> EERKKELAKEVIETA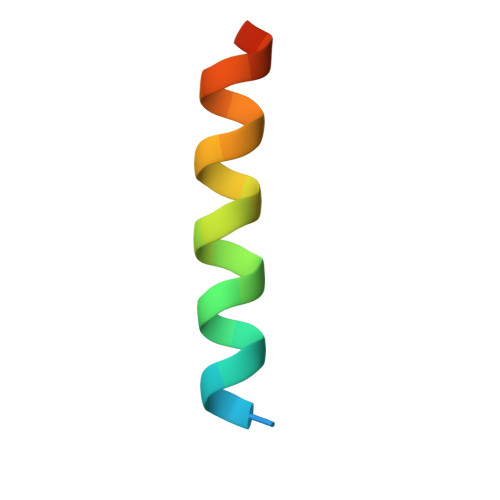KKLIEKLAKEE> NSELDRLSKDDRNWVMQTKDYSATHFSRLTEINSHNVKNLKVAWTLSTGTLHGHEGAPLVVDGIMYIHT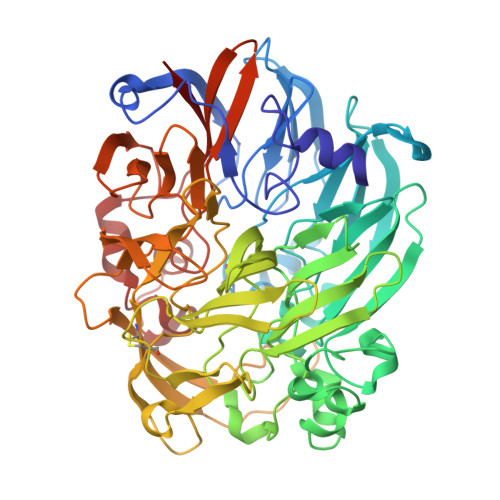PFPNNVYAVDLNDTRKMLWQYKPKQNPAARAVACCDVVNRGLAYVPAGEHGPAKIFLNQLDGHIVALNAKTGEEIWKMENSDIAMGSTLTGAPFVVKDKVLVGSAGAELGVRGYVTAYNIKDGKQEWRAYATGPDEDLLLDKDFNKDNPHYGQFGLGLSTWEGDAWKIGGGTNWGWYAYDPKLDMIYYGSGNPAPWNETMRPGDNKWTMTIWGRDADTGRAKFGYQKTPHDEWDYAGVNYMGLSEQEVDGKLTPLLTHPDRNGLVYTLNRETGALVNAFKIDDTVNWVKKVDLKTGLPIRDPEYSTRMDHNAKGICPSAMGYHNQGIESYDPDKKLFFMGVNHICMDWEPFMLPYRAGQFFVGATLNMYPGPKGMLGQVKAMNAVTGKMEWEVPEKFAVWGGTLATAGDLVFYGTLDGFIKARDTRTGELKWQFQLPSGVIGHPITYQHNGKQYIAIYSGVGGWPGVGLVFDLKDPTAGLGAVGAFRELAHYTQMGGSVFVFSL({[(2R)-2-{[(4-ethyl-2,3-dioxopiperazin-1-yl)carbonyl]amino}-4-(4-hydroxyphenyl)butanoyl]amino}methyl)boronic acid | C18 H25 B N4 O7 | 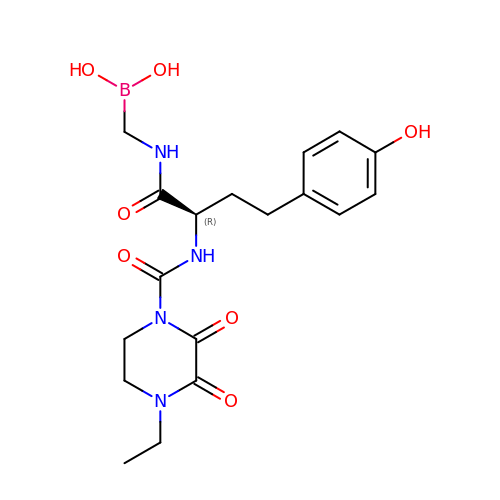RSVZQUMTCHOFDU-CQSZACIVSA-N> VVGGTEAQRNSWPSQISLQYRSGSSWAHTCGGTLIRQNWVMTAAHCVDRELTFRVVVGEHNLNQNDGTEQYVGVQKIVVHPYWNTDDVAAGYDIALLRLAQSVTLNSYVQLGVLPRAGTILANNSPCYITGWGLTRTNGQLAQTLQQAYLPTVDYAICSSSSYWGSTVKNSMVCAGGDGVRSGCQGDSGGPLHCLVNGQYAVHGVTSFVSRLGCNVTRKPTVFTRVSAYISWINNVIASN;> PCTL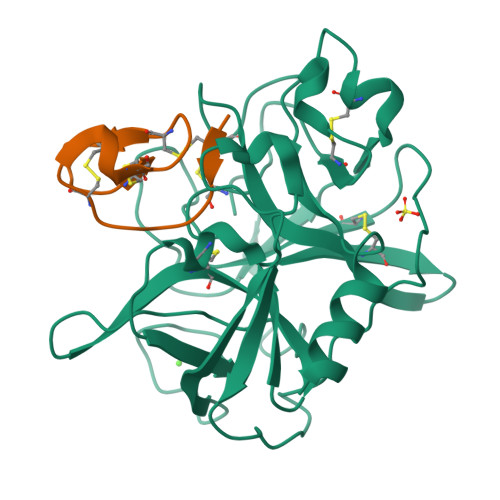EYMRCKQDSDCLAGCVCGPNGFCG> ELTPDQQTLLHFIMDSYNKQRMPQEITNKILKEEFSAEENFLILTEMATNHVQVLVEFTKKLPGFQTLDHEDQIALLKGSAVEAMFLRSAEIFNKKLPSGHSDLLEERIRNSGISDEYITPMFSFYKSIGELKMTQEEYALLTAIVILSPDRQYIKDREAVEKLQEPLLDVLQKLCKIHQPENPQHFACLLGRLTELRTFNHHHAEMLMSWRVNDHKFTPLLCEIWDVQ;> NEALLRYLL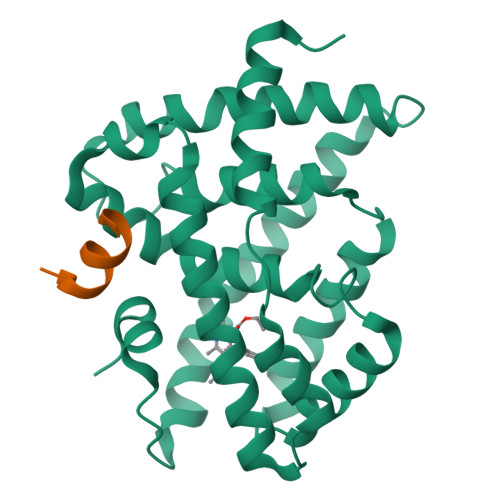DK> ADPSEHCSHMIGNGHLKVLQQLIDSQMETSCQIAFEFVDQEQLDDPVCYL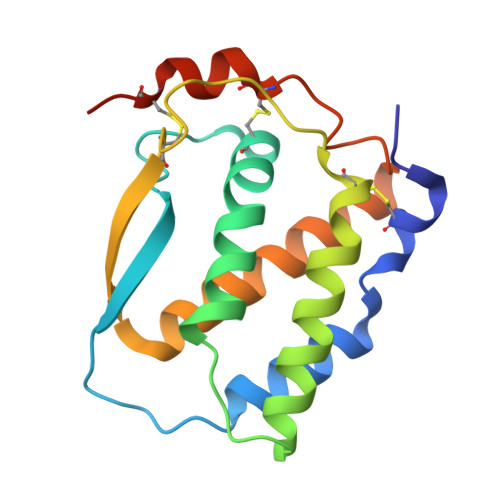KKAFFLVQDIIDETMRFKDNTPNANATERLQELSNNLNSCFTKDYEEQNKACVRTFHETPLQLLEKIKNFFNETKNLLEKDWNIFTKNCNNSFAKCSSHHHHHHH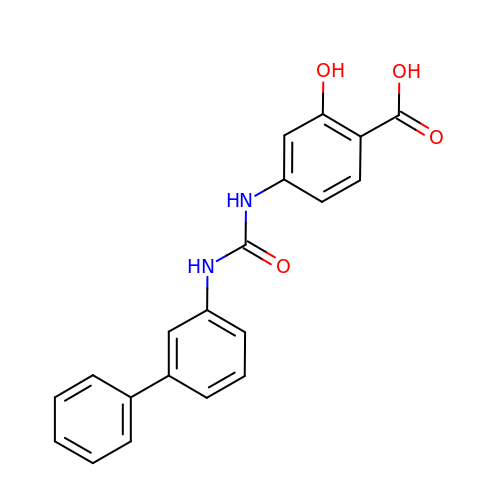4-{[([1,1'-biphenyl]-3-yl)carbamoyl]amino}-2-hydroxybenzoic acid | C20 H16 N2 O4 | FJUJZHPFSHEAMU-UHFFFAOYSA-N>GMNKEVDLSVSCLGKVKELKYDVIILPWGATEPHNLHLPYLTDCILPHDIAVEAAELALSRSGVRC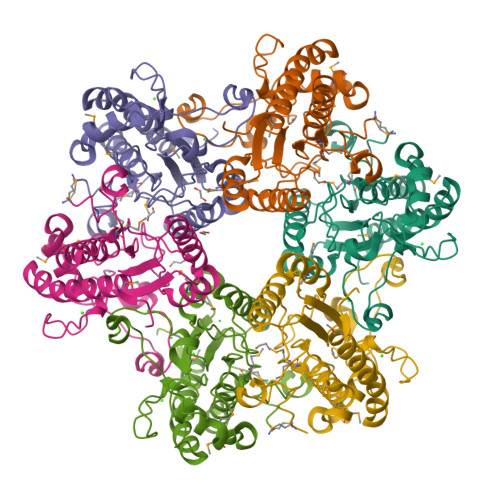MVMPPVPFGAHNPGQRELPFCIHTRYATQQAILEDIVSSLHVQGFRKLLILSGHGGNNFKGMIRDLAFEYPDFLIAAANWFEVVSPKGYFEAEIDDHAGESETSVMMHYHPELVNLAEAGDGESKPFAIASLNEKVAWVPRHWDKATVDSGVGNPKKATAEKGERYVKPIVEKLAGLFEEMAQHDLYE[12x]>[2x]MGSSHHHHHHSSGLVPRGSMSTSWSDRLQNAADMPANMDKHALKKYRREAYHRVFVNRSLAMEKIKCFGFDMDYTLAVYKSPEYESLGFELTVERLVSIGYPQELLSFAYDSTFPTRGLVFDTLYGNLLKVDAYGNLLVCAHGFNFIRGPETREQYPNKFIQRDDTERFYILNTLFNLPETYLLACLVDFFTN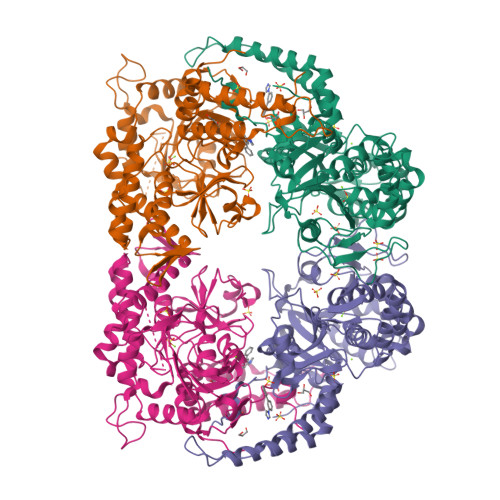CPRYTSCETGFKDGDLFMSYRSMFQDVRDAVDWVHYKGSLKEKTVENLEKYVVKDGKLPLLLSRMKEVGKVFLATNSDYKYTDKIMTYLFDFPHGPKPGSSHRPWQSYFDLILVDARKPLFFGEGTVLRQVDTKTGKLKIGTYTGPLQHGIVYSGGSSDTICDLLGAKGKDILYIGDHIFGDILKSKKRQGWRTFLVIPELAQELHVWTDKSSLFEELQSLDIFLAELYKHLDSSSNERPDISSIQRRIKKVTHDMDMCYGMMGSLFRSGSRQTLFASQVMRYADLYAASFINLLYYPFSYLFRAAHVLMPHESTVEHTHVDINEMESPLATRNRTSVDFKDTDYKRHQLTRSISEIKPPNL> GLPTLATPGSNQFLTSDDFQSPSAMPQFDVTPEMDIPGQVNNLMEIAEVDSVVPVNNTEGKEMSIEAYQIPVQSNPTNGSQVFGFPLTPGASSVLNRTLLGEILNYYAHWSGSIKLTFMFCGSAMATGKFLLAYSPPGAGAPTTRKEAMLGTHVIWDVGLQS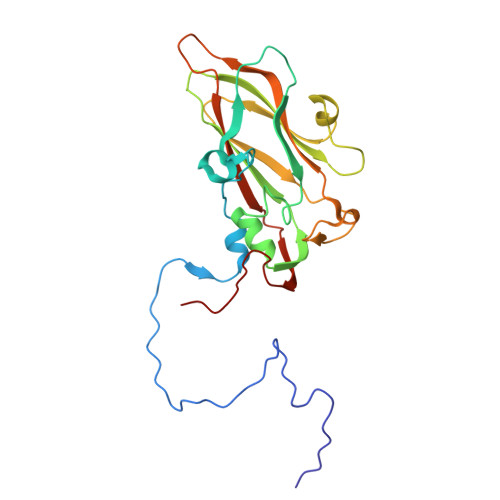SCVLCIPWISQTHYRYVVMDEYTAGGYITCWYQTNIVVPADAQSDCKILCFVSACNDFSVRMLKDTPFIKQDNFFQ> MENLNHCPLEDIKVNPWKTPQSTARVITLRVEDPNEI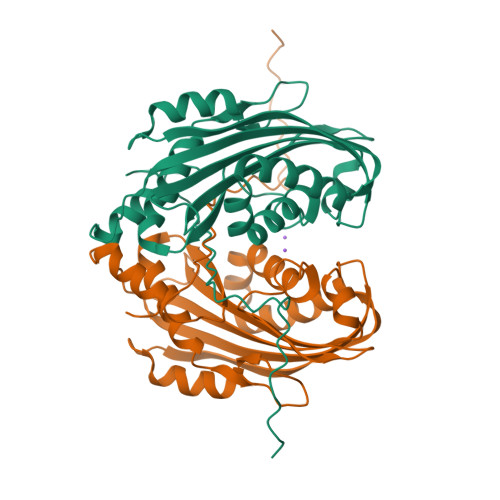NNLLSINEIDNPNYILQAIMLANAFQNALVPTSTDFGDALRFSMPKGLEIANTITPMGAVVSYVDQNVTQTNNQVSVMINKVLEVLKTVLGVALSGSVIDQLTAAVTNTFTNLNTQKNEAWIFWGKETANQTNYTYNVLFAIQNAQTGGVMYCVPVGFEIKVSAVKEQVLFFTIQDSASYNVNIQSLKFAQPLVSSSQYPIADLTSAINGTL>XEWEAIEKKIAANESKDQAIEKKIQAIEK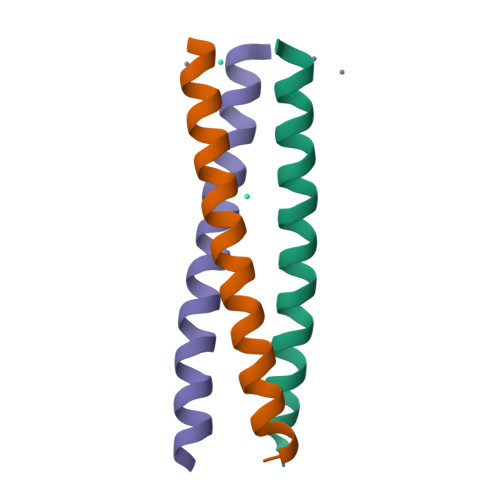KIEAIEHGX[3x]>[4x]SNAMKIVKRALTFEDVLLRPGYSEVLPKEVKIHTKLTKNITLNMPLISAAMDTVTEHRAAIMMARLGGLGVIHKNMDIASQVREVKRVKKSESGGIKDLKKRK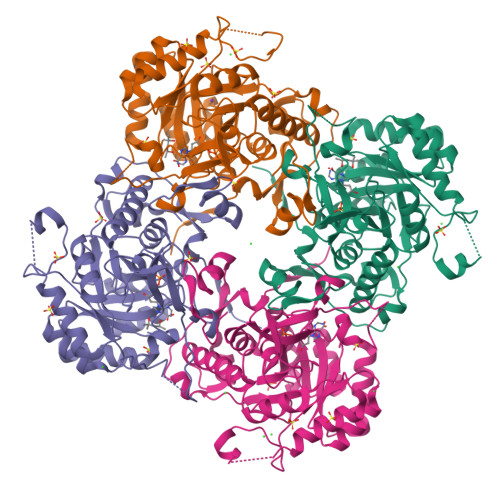EYPDANKDNFGRLRVGAAIGVGQMDRVDALVEAGVDVVVLDSAHGHSKGIIDTVKAIKAKYPNLDLIAGNIATAAAAKALCEAGVDAVKVGIGPGSICTTRIVSGVGVPQISAIDECVEEANKFGVPVIADGGIKYSGDIAKALAVGASSVMIGSLLAGTDESPGELFTYQGRQYKSYRGMGSLGAMQKGSSDRYFQQGTAQDKLVPEGIEGRVPYVGSIRSVVHQLLGGLRSSMGYVGAKDIEDFQKRAEFVEITTAGLKESHVHDVTITHEAPNYKVNHQ> MRGSHHHHHHGSLMPGGKEFYNFYPEYVVGLQWMGDNYVFIEGDDLVFNKANGKSAQTTRFSAADLNALMPEGCKFQTTDAFPSFRTLDAGRGLVVLFTQGGLVGFDMLARKVTYLFDTNEETASLDFSPVGDRVAYVRNHNLYIARGGKLGEGMSRAIAVTIDGTETLVYGQAVHQREFGIEKGTFWSPKGSCLAFYRMDQSMVKPTPIVDYHPLEAESKPLYYPMAGTPSHHVTVGIYHLATGKTVYLQTGEPKEKFLTNLSWSPDENILYVAEVNRAQNECKVNAYDAETGRFVRTLFVETDKHYVEPLHPLTFLPGSNNQFIWQSRRDGWNHLYLYDTTGRLIRQVTKGEWEVTNFAGFDPKGTRLYFESTEASPLERHFYCIDIKGGKTKDLTPESGMHRTQLSPDGSAIIDIFQSPTVPRKVTVTNIGKGSHTLLEAKNPDTGYAMPEIRTGTIMAADGQTPLYYKLTMPLHFDPAKKYPVIVYVY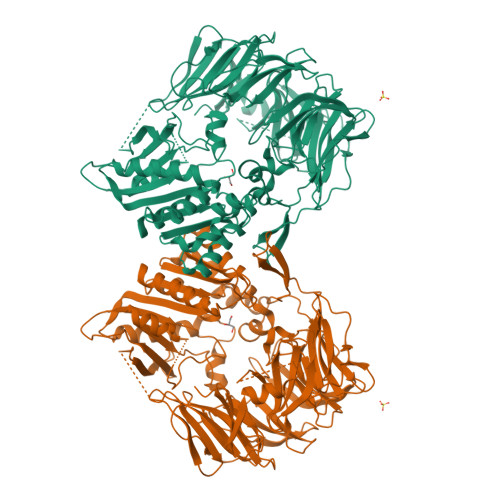GGPHAQLVTKTWRSSVGGWDIYMAQKGYAVFTVDSRGSANRGAAFEQVIHRRLGQTEMADQMCGVDFLKSQSWVDADRIGVHGWSYGGFMTTNLMLTHGDVFKVGVAGGPVIDWNRYAIMYGERYFDAPQENPEGYDAANLLKRAGDLKGRLMLIHGAIDPVVVWQHSLLFLDACVKARTYPDYYVYPSHEHNVMGPDRVHLYETITRYFTDHL> MKIICNQKILANRIGIAQKAINGKTTIELLKGILISTEEGQLKLTGYDAEIGIETYVQAEIIEKGDVVVDARLFGDIIRKLPDSFVEIETDSENNIYINCVNSRFKIKGYAAKEFPKLPELNEEDLYSIPQEILKNMIKQTVFAISQDQTKPVLMGELLEIVDRNLNLVAIDGYRLAVKSCSVDSLTENIKVIIPGKTLID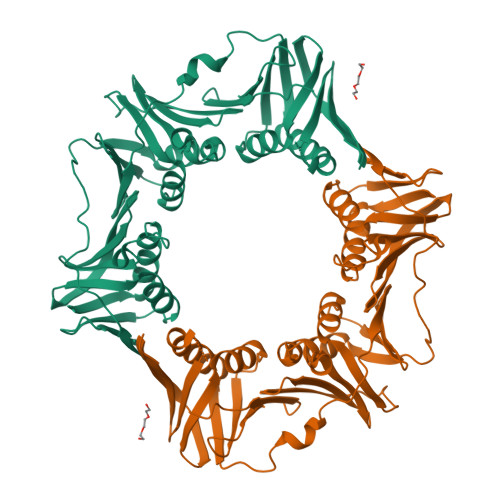VNSLLSGEDNVKVGFNEKNAIFIINDTKIITRLLEGDFIDYKKLLPREHNSRVKLNTKELLNSIERASLLSQSEKNNLIKLSIRDKVMAITSNTEKGNVYEEVEIDLDGDYLDIAFNSRYFIEGLKNIDNEEIFIEFTTNVNPCIIKPTDDVNYIYLLLPVRISSNI> MFKNAKEFVQYANKLKTLREKKLNGVSIYVCVGTGCTAKGALKVYSAFEEELKKRNLLGQVTLEKIDDDKVTLNRTGCCGRCSSGPLVKIMPYRFFYSNVAPEDVPEIVDRTVLKGEPIERLFLTDPLTGEKVPRIEDTTLFKNQDFYIMEAIGESECDSIEDYIARSGYESLVKALTSMTPEEIIETVKASGLRGRGGGGFPTGLKWEFTRKAQGDIKFVVCNGDEGDPGAFMNRTLLERDPHLVLEGMIIAGYAVGAQKGYAYIRAEYPFAVKMFKKAIEDARKLGLLGENILGTGFSFDLEVKEGAGAFVCGEETALLASIEGKRGMPRPKPPFPAQSGLWGKPTLINNVETYANIPRILRDGVENYRKRGTENSPGTKMFSVAGPLKATGIIEVEFGTTLRDIIYNICGGFVEGEEFKAVQIGGPSGACLSEDFI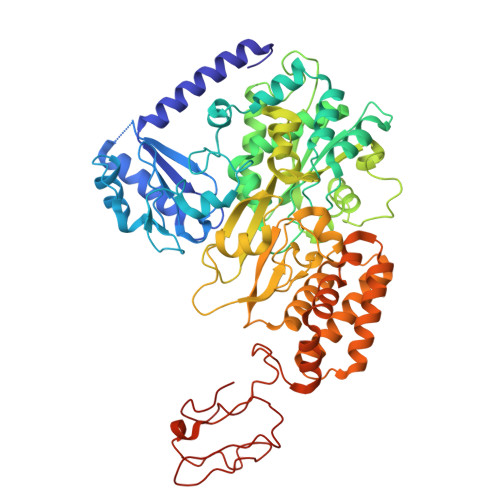DMPLDYDTLKKADAMVGSGGIVVITKKTCMVEVARFFLDFTKRESCGKCVPCREGTMQAYNILEKFTHGKATYEDLKTLEHLSKTIKTASLCGLGKTAPNPILSTLKLFREEYIAHIEGECPSGMCTAFKKYVINPDICKGCGLCARSCPQNAITGERGKPYTIDQEKCVKCGLCASKCPFKAIELV> MGIDINTKIFNSVAEVFQKAQGSYAGHRKHIAVLKKIQSKAVEQGYEDAFNFWFDKLVTKILPLKKNEIIGDRIVKLVAAFIASLERELILAKKQNYKLTNDEEGIFSRFVDQFIRHVLRGVESPDKNVRFRVLQLLAVIMDNIGEIDESLFNLLILSLNKRIYDREPTVRIQAVFCLTKFQDEEQTEHLTELSDNEENFEATRTLVASIQNDPSAEVRRAAMLNLINDNNTRPYILERARDVNIVNRRLVYSRILKSMGRKCFDDIEPHIFDQLIEWGLEDRELSVRNACKRLIAHDWLNALDGDLIELLEKLDVSRSSVCVKAIEALFQSRPDILSKIKFPESIWKDFTVEIAFLFRAIYLYCLDNNITEMLEENFPEASKLSEHLNHYILLRYHHNDISNDSQSHFDYNTLEFIIEQLSIAAERYDYSDEVGRRSMLTVVRNMLALTTLSEPLIKIGIRVMKSLSI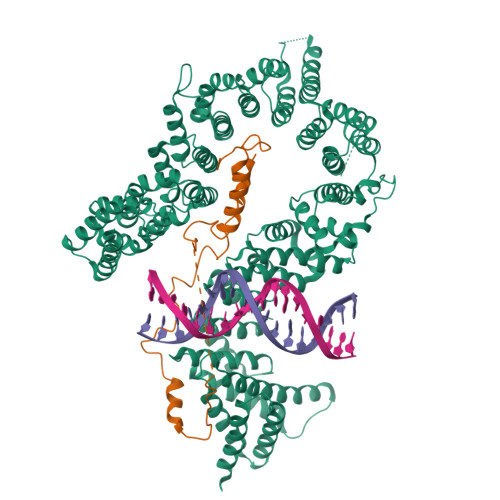NEKDFVTMAIEIINDIRDDDIEKQESESDIINNLPPEKEASSATIVLCLTRSSYMLELVNTPLTENILIASLMDTLITPAVRNTAPNIRELGVKNLGLCCLLDVKLAIDNMYILGMCVSKGNASLKYIALQVIVDIFSVHGNTVVDGEGKVDSISLHKIFYKVLKNNGLPECQVIAAEGLCKLFLADVFTDDDLFETLVLSYFSPINSSNEALVQAFAFCIPVYCFSHPAHQQRMSRTAADILLRLCVLWDDLQSSVIPEVDREAMLKPNIIFQQLLFWTDPRNLVNQTGSTKKDTVQLTFLIDVLKIYAQIEKKEIKKMIITNINAIFLSSEQDYSTLKELLEYSDDIAENDNLDNVSKNALDKLRNNLNSLIEEINERSETQTKDENNTANDQYSSILGN;> GPLGHMSIFEKDLMAYFDENLNRNWRGREHWKVRNFKKANKSMDTKKKHKQKKVLEIDFFKTDDSFEDKVFASKGRTKIDMPIKNRKNDTHYLLPDDFHFSTDRITRLFIKPGQKMSLFSHRKHT>MTHRKQPSSSSKLPDSILKRGAEASKVLEEHLERGNIIRIISHNDADGLSAAGVVARAISSMNGQFHISILSRLKKEFIKKLSGEKYSLFFFCDMGSAYLEEISRLKGDVIVADHHQPSESEAGPHVVHINPHLHGLDGSRDLSASGTAYLATRLLNRKTAPLALVGALGDMQYTDGFTGANRFIMEEAVEEGVLQVHSDLKLASRYTEPLYRSIAYTFNPALPGLTGDMEASMGFLENIGVSYGVKYPDLSPEERDVLRDELTRINPEIFGEVFTSREFRNIGDLSDIAGVLDACGKNRKYGIGIGLCLGEREGALDVALELQKNYREELVKGLAWIRREGSTTLENLQYIYSEDKAFKGIMGTIASISLSLKILDPDIPLLGLSRMDQHVKVSARTTRPAV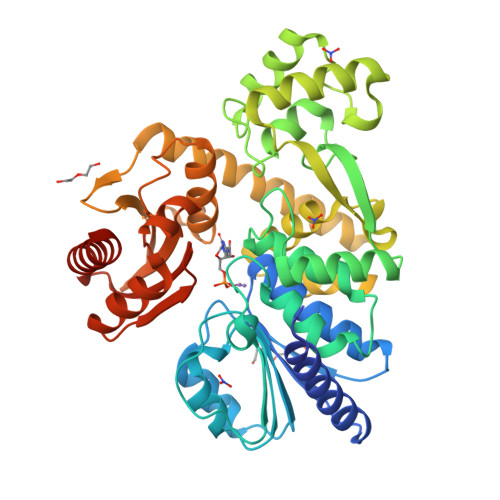ERGVNLGVALRDAAASFGGTGGGHDIAAGAMVPYRDMESFLQLVDEILGTQTGPAENLYFQ[2x]> GSFTMASMTGGQQMGRGSMNGDVQSVIRGYLERAQVAKTMSDAGRWNEAGDLLRQLMTDVKSCKISASNRDEHDARNTFLRALEANLKLVQQNVRDEDDLHE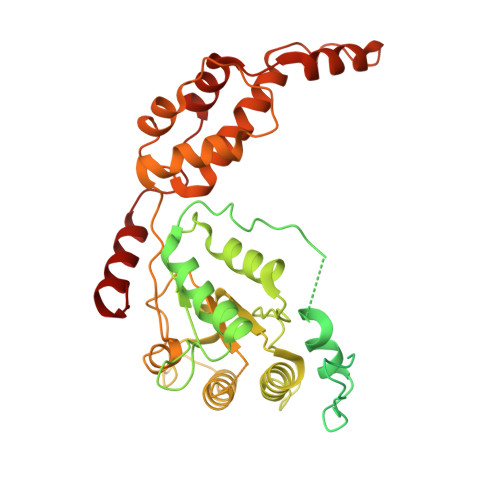AMTRQSGSPEPPADPDVWSKPSPPLPSSSKFGATKKGVGAAGPRPREISKSTSSMSTNPADVKPANPTQGILPQNSAGDSFDASAYDAYIVQAVRGTMATNTENTMSLDDIIGMHDVKQVLHEAVTLPLLVPEFFQGLRSPWKAMVLAGPPGTGKTLIARAIASESSSTFFTVSSTDLSSKWRGDSEKIVRLLFELARFYAPSIIFIDQIDTLGGQRGNSGEHEASRRVKSEFLVQMDGSQNKFDSRRVFVLAATNIPWELDEALRRRFEKRIFIPLPDIDARKKLIEKSMEGTPKSDEINYDDLAARTEGFSGADVVSLCRTAAINVLRRYDTKSLRGGELTAAMESLKAELVRNIDFEAALQAVSPSAGPDTMLKCKEWCDSFGAM4-[(6-chloropyridin-2-yl)sulfamoyl]benzene-1-sulfonic acid | 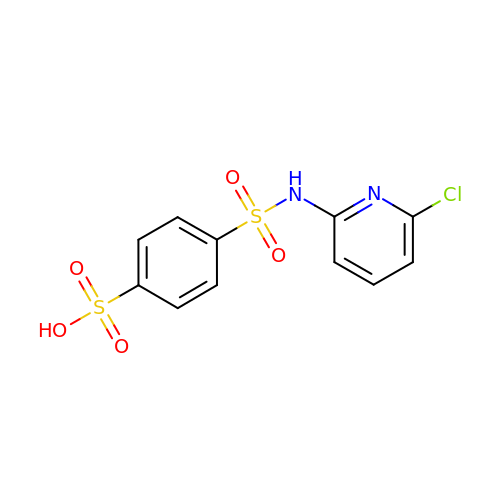C11 H9 Cl N2 O5 S2 | AOXDXPJHIZMZOS-UHFFFAOYSA-N> GSHMASMLLDTFQGYNAYSSALGEYAKQKNIDQVENIILSQWSFFFDEEQFYKNQWYTGAADGPVDVVLNEDLRNFAN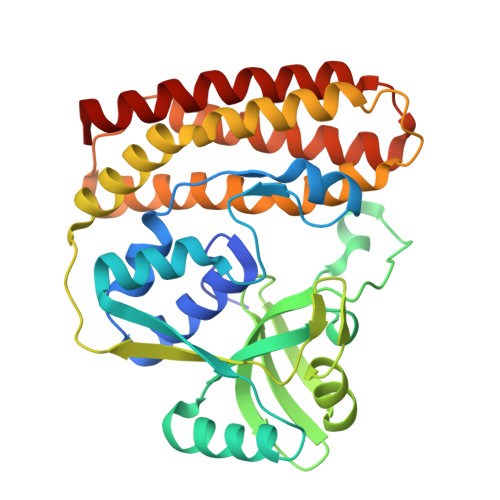IEVLEHISSESQAIDEGRKVLEKHGLQIVLMDFYYMNSFNWKSLSRFNVTREHDPHFAVLTQINENSVHIIDPYYHHEENMSMEDFIKSRNSMTKQGKISFNSYEIFSNGTKKSNIKELLYYRFNRYLQEKMFGKITQFGQVVKKQLDNKDRKWAFTGYNCLNSVVYQHQNLINLQKKFSLEMPPNLQELLDNWALIRKKLFEYYSRGSYNTEEISNLICKVASSEEQFAQEVLKVL Unphosphorylated STATs form an anti-parallel dimer/monomer equilibrium, and upon efficient recruitment to the cognate receptor–kinase complex, are phosphorylated on a specific tyrosine residue, which promotes parallel dimerization by conformational rearrangement. The activated STAT dimer translocates to the nucleus, initiating transcription of target genes and altering chromatin involved in loop formation in enhancer-promoter landscapes. The canonical domains of the STAT family are all present with the coiled-coil domain (CCD, S138-T331), DNA-binding domain (DBD, F332-V470), linker domain (H471-D591), and SH2 domain (Q592-P685). Archetypical STAT-type SH2 domains are comprised of an anti-parallel β-sheet created by three β-strands (conventionally labeled βB-βD) surrounded by three α-helices (αA, αB’, and αB), which are also observed in STAT5B.

Notably, STAT5BN642H was identified and validated as a severe oncogenic driver mutation. To investigate whether STAT5BN642H perturbs the protein structure, we crystalized the mutant using the same domain boundaries as the  wild-type protein (A136-Q703). The crystal structure of STAT5BN642H was solved to 3.21 Å with a similar space group to the wild-type protein. The βD strand containing N642H was observed with excellent electron density and showed two distinct conformations. In one STAT5BN642H conformation, the βD strand associates securely with the βC strand forming additional H-bonding partners, not observed in the wild-type conformation, thereby fully completing the anti-parallel β-sheet. In this conformation, the H642 likely coordinates the phosphate, similar to that observed in other SH2 domains such as Src and phosphatidylinositol-4,5-bisphosphate 3-kinase (PI3K). The second conformation showed the N642-containing βD strand dissociated from the βC and βB strands, resulting in an incomplete β-sheet. This partially completed β-sheet places the SH2 domain in an open, potentially inactivated, state. Alternatively, it is also possible that this conformation is more capable of activating STAT5B either through facilitating interactions with the C-terminal region and dimer interface or providing greater access to the pY pocket to increase phospho-ligand association kinetics. Notably, the affinity of the phospho-peptide with the full-length STAT5BN642H (Kd = 15 ± 1 nM) was ~6–7-fold higher than wild-type (Kd = 102 ± 11 nM).

>[2x]STGSAMSQKHLQINQTFEELRLVTQDTENELKKLQQTQEYFIIQYQESLRIQAQFGPLAQLSPQERLSRETALQQKQVSLEAWLQREAQTLQQYRVELAEKHQKTLQLLRKQQTIILDDELIQWKRRQQLAGNGGPPEGSLDVLQSWCEKLAEIIWQNRQQIRRAEHLCQQLPIPGPVEEMLAEVNATITDIISALVTSTFIIEKQPPQVLKTQTKFAATVRLLVGGKLNVHMNPPQVKATIISEQQAKSLLKNENTRNDYSGEILNNCCVMEYHQATGTLSAHFRNMSLKRIKRSDRRGAESVTEEKFTILFESQFSVGGNELVFQVKTLSLPVVVIVHGSQDNNATATVLWDNAFAEPGRVPFAVPDKVLWPQLCEALNMKFKAEVQSNRGLTKENLVFLAQKLFNNSSSHLEDYSGLSVSWSQFNRENLPGRNYTFWQWFDGVMEVLKKHLKPHWNDGAILGFVNKQQAHDLLINKPDGTFLLRFSDSEIGGITIAWKFDSQERMFWHLMPFTTRDFSIRSLADRLGDLNYLIYVFPDRPKDEVYSKYYTPVPCESATAKAVDGYVKPQ> IINGEDCSPHSQPWQAALVMENELFCSGVLVHPQWVLSAAHCFQNSYTIGLGLHSLEADQEPGSQMVEASLSVRHPEYNRPLLANDLMLIKLDESVSESDTIRSISIASQCPTAGNSCLVSGWGLLANGRMPTVLQCVNVSVVSEEVCSKLYDPLYHPSMFCAGGGQDQKDSCNGDSGGPLICNGYLQGLVSFGKAPCGQVGVPGVYTNLCKFTEWIEKTVQA;> SSVVVDTNG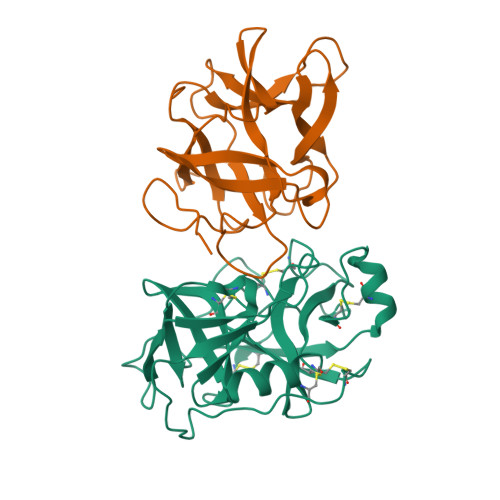QPVSNGADAYYLVPVSHGHAGLALAKIGNEAEPRAVVLDPHHRPGLPVRFESPLRINIIKESYFLNIKFGPSSSDSGVWDVIQQDPIGLAVKVTDTKSLLGPFKVEKEGEGYKIVYYPERGQTGLDIGLVHRNDKYYLAVKDGEPCVFKIRKATDE BILIVERDIN IX GAMMA CHROMOPHORE | C33 H34 N4 O6 | 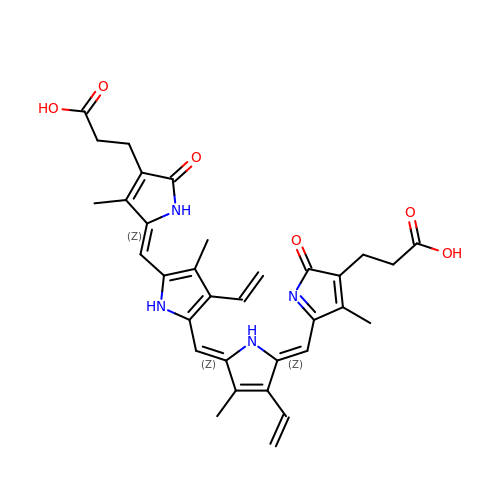ISQGGWQAVOHBFX-BGSBWKAWSA-N N-[1-(3-METHYLBUTYL)PIPERIDIN-4-YL]-N-{4-[METHYL(PYRIDIN-4-YL)AMINO]BENZYL}-4-PENTYLBENZAMIDE | C35 H48 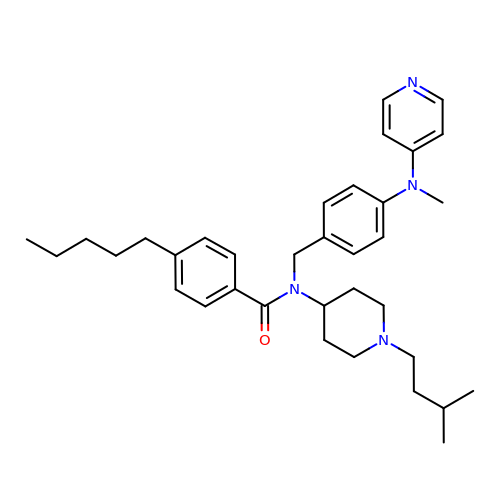N4 O | WRFRQUOWNCJODU-UHFFFAOYSA-N>[2x]DPM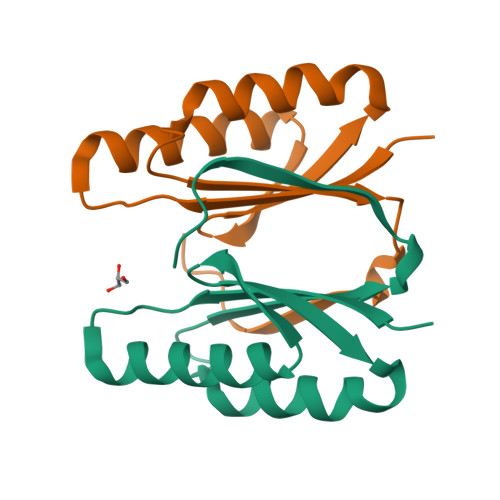FIIVCYDVETITQEGRARLRKVAKTCESHGQRVQKSVFECQLEPADYLQFEAKLSKIINSKTDNLRIYSLDAISVSKIKQFGVSNILDF> GSNDLGSKSEIRKEENGNVTIITQNNKQIRKYSSTDSATTKSNSKITVDASFVDDKFSSEMTTIISLKGFIPSGRKIFALSKYRGVMRWPIKYMVDLKNNSLDSSVKIVDSVPKNTISTKEVNNTISYSIGGGIDTSNKASLNANYAVSKSISYVQPDYNTIQTNDTNSIASWNTEFAETRDGYNVNSWNIVYGNQMFMRSRYSGTSTTNFTPDYQLSSLITGGFSPNFGVVLTAPNGTKKSQIEISLKREINSYHIAWDTEWQGRNYPDSKIEETVKFELDWEKHTIRQISHHHHHH

Clostridium perfringens Delta toxin is one of the three hemolysin-like proteins produced by C. perfringens type C and possibly type B strains. Delta toxin itself is cytotoxic to the wide range of human and animal macrophages and platelets that present GM2 ganglioside on their membranes. It has sequence similarity with Staphylococcus aureus β-pore forming toxins and is expected to heptamerize and form pores in the lipid bilayer of host cell membranes. Subsequently, they oligomerize on the cell surface to form prepores that insert amphipathic hairpins into the lipid bilayer to form an oligomeric β-barrel pore.

Here, we present the monomeric structure of Delta toxin at 2.4 Å resolution, determined by X-ray crystallography. It includes a monomer of Delta toxin, comprising 282 residues (residues Ile9 to Ser290), 139 water molecules, three glycerol molecules, one imidazole and three zinc molecules. C. perfringens Delta toxin structure has an elongated ellipsoid shape composed of eighteen β-strands and three short helical fragments: two 310 helices and one α-helix. These secondary structure elements are arranged into three structural domains: a β-sandwich domain, a stem domain and a rim domain. In Delta toxin, the N-terminal residues form a β-hairpin that extends halfway along the β-sandwich domain and creates a cap above the folded, monomeric stem domain residues. Finally, Delta toxin has a four-residue deletion in the residue 177–183 loop relative to the S. aureus proteins. This deletion means that Delta toxin does not possess a Tryptophan (residue 177 in LukF) that is important for phosphatidylcholine binding in the S. aureus proteins. There are three glycerol molecules bound to the hydrophobic region of the rim domain. Interestingly, when Delta toxin and LukF are superposed, the glycerol of Delta toxin is positioned where the glycerol moiety of the phosphatidylcholine would be expected to be in the LukF structure, if it had been ordered. One of the glycerol molecules in the Delta toxin structure is interacting with the Arg200 residue, and, it is likely that, in analogy with these related proteins, Arg200 in Delta toxin is important for cell surface recognition.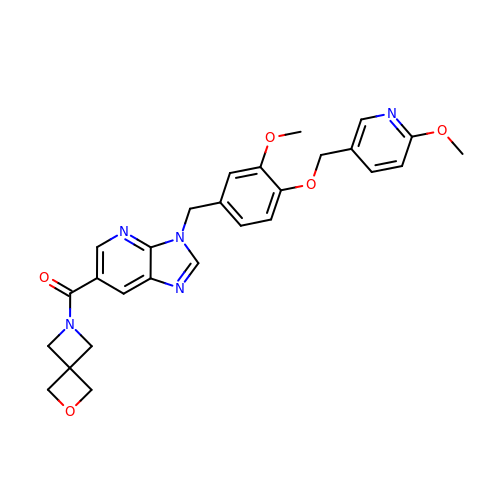[3-({3-methoxy-4-[(6-methoxypyridin-3-yl)methoxy]phenyl}methyl)-3H-imidazo[4,5-b]pyridin-6-yl](2-oxa-6-azaspiro[3.3]heptan-6-yl)methanone | C27 H27 N5 O5 | GGMUAMIMZXIUOT-UHFFFAOYSA-N>[2x]MAMQAAKRANIRLPPEVNRILMIRNLPYKITAEEMYDIFGKYGPIRQIRVGNTPETRGTAYVVYEDIFDAKNACDHLSGFNVCNRYLVVLYYNANRAFQ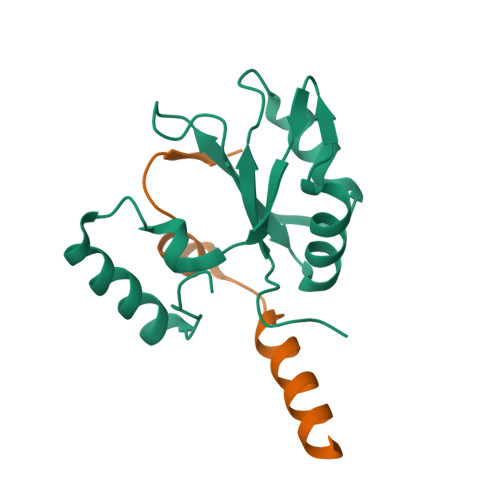KMDTKKKEEQLKLLKEKYGINTDPPK;>GEQLQAWRWEREIDERNRPLSDEELDAMFPEGYKVL[2x]> SMGTRPRRKKHDYRIALFGGSQPQSCRYFNPKDYSWTDIRCPFEKRRDAACVFWDNVVYILGGSQLFPIKRMDCYNVVKDSWYSKLGPPTPRDSLAACAAEGKIYTSGGSEVGNSALYLFECYDTRTESWHTKPSMLTQRCSHGMVEANGLIYVCGGSLGNNVSGRVLNSCEVYDPATETWTELCPMIEARKNHGLVFVKDKIFAVGGQNGLGGLDNVEYYDIKLNEWKMVSPMPWKGVTVKCAAVG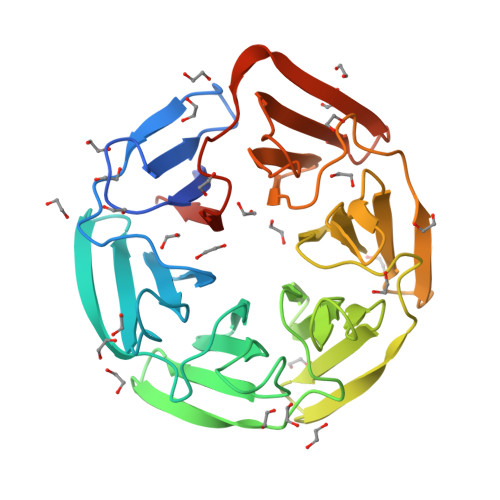SIVYVLAGFQGVGRLGHILEYNTETDKWVANSKVRAFPVTSCLICVVDTCGANEETLET> PSSEQAWLEDAQVFIQKTLCPAVKEPNVQLTPLVIDCVKTVWLSQGRNQGSTLPLSYSFVSVQDLKTHQRLPCCSHLSWSSSAYQAWAQEAGPNGNPLPREQLLLLGTLTDLSADLEQECRNGSLYVRDNTGVLSCELIDLDLSWLGHLFLFPRWSYLPPARWNSSGEGHLELWDAPVPVFPLTISPGPVTPIPVLYPESASCLLRLRNKLRGVQRNLAGSLVRLSALVKSKQKAYFILSLGRSHPAVTHVSIIVQVPAQLVWHRALRPGTAYVLTELRVSKIRGQRQHVWMTSQSSRLLLLKPECVQELELELEGPLLEADPKPLPMPSNSEDKKDPESLVRYSRLLSYSGAVTGVLNEPAGLYELDGQLGLCLAYQQFRGLRRVMRPGVCLQLQDVHLLQSVGGGTRRPVLAPCLRGAVLLQ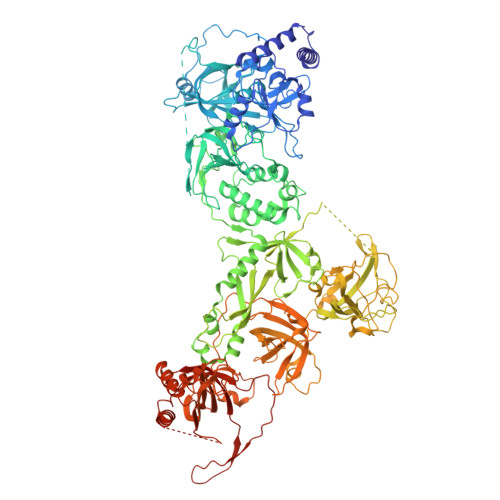SFSRQKPGAHSSRQAYGASLYEQLVWERQLGLPLYLWATKALEELACKLCPHVLRHHQFLQHSSPGSPSLGLQLLAPTLDLLAPPGSPVRNAHNEILEEPHHCPLQKYTRLQTPSSFPTLATLKEEGQRKAWASFDPKALLPLPEASYLPSCQLNRRLAWSWLCLLPSAFCPAQVLLGVLVASSHKGCLQLRDQSGSLPCLLLAKHSQPLSDPRLIGCLVRAERFQLIVERDVRSSFPSWKELSMPGFIQKQQARVYVQFFLADALILPVPRPCLHSATPSTPQTDPTGPEGPHLGQSRLFLLCHKEALMKRNFCVPPGASPEVPKPALSFYVLGSWLGGTQRKEGTGWGLPEPQGNDDNDQKVHLIFFGSSVRWFEFLHPGQVYRLVAPGPATPMLFEKDGSSCISRRPLELAGCASCLTVQDNWTLELESSQDIQDVLDANKSLPESSLTDLLSDNFTDSLVSFSAEILSRTLCEPLVASLWMKLGNTGAMRRCVKLTVALETAECEFPPHLDVYIEDPHLPPSLGLLPGARVHFSQLEKRVSRSHNVYCCFRSSTYVQVLSFPPETTISVPLPHIYLAELLQGGQSPFQATASCHIVSVFSLQLFWVCAYCTSICRQGKCTRLGSTCPTQTAISQAIIRLLVEDGTAEAVVTCRNHHVAAALGLCPREWASLLDFVQVPGRVVLQFAGPGAQLESSARVDEPMTMFLWTLCTSPSVLRPIVLSFELERKPSKIVPLEPPRLQRFQCGELPFLTHVNPRLRLSCLSIRESEYSSSLGILASSC>CSLIPDYQRPEAPVAAAYPQGQAYGQNTGAAAVPAADIGWREFFRDPQLQQLIGVALENNRDLRVAALNVEAFRAQYRIQRADLFPRIGVDGSGTRQRLPGDLSTTGSPAISSQYGVTLGTTAWELDLFGRLRSLRDQALEQYLATEQAQRSAQTTLVASVATAYLTLKADQAQLQLTKDTLGTYQKSFDLTQRSYDVGVASALDLRQAQTAVEGARATLAQYTRLVAQDQNALVLLLGSGIPANLPQGLGLDQTLLTEVPAGLPSDLLQRRPDILEAEHQLMAANASIGAARAAFFPSISLTANAGTMSRQLSGLFDAGSGSWLFQPSINLPIFTAGSLRASLDYAKIQKDINVAQYEKAIQTAFQEVADGLAARGTFTEQLQAQRDLVKASDEY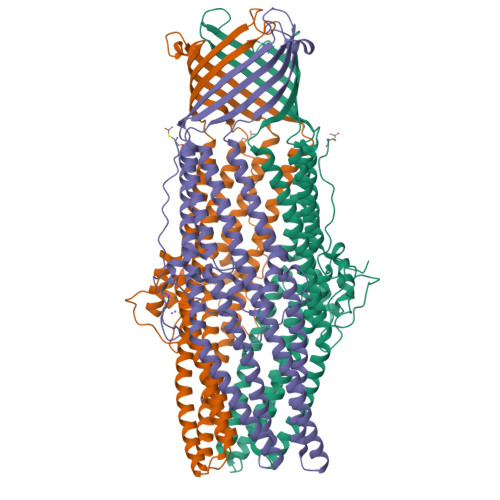YQLADKRYRTGVDNYLTLLDAQRSLFTAQQQLITDRLNQLTSEVNLYKALGGGWNQQTVTQQQTAKKEDPQAHHHHHH[3x]> A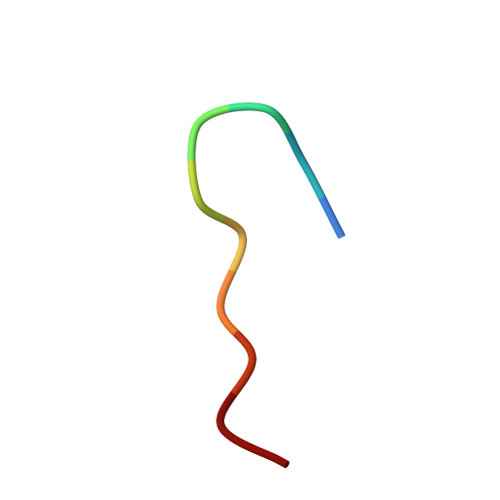AKAAAAAAA> MENDPNLFVALY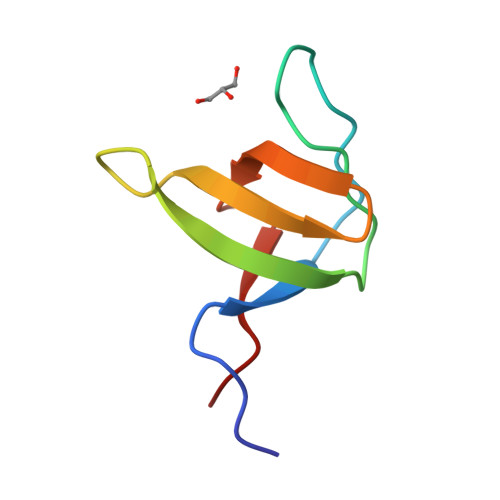DFVASGDNTLSITKGEKLRVLGYNHNGEWCEAQTKNGQGWVPSAYITPVNS>[4x]MKHHHHHHHHGGLVPRGSHG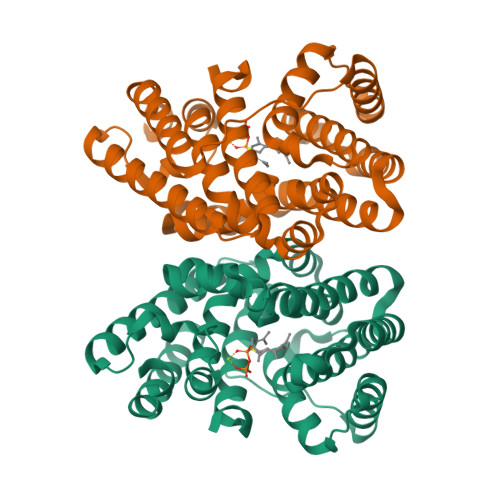GSEFMTTGLSTAGAQDIGRSSVRPYLEECTRRFQEMFDRHVVTRPTKVELTDAELREVIDDCNAAVAPLGKTVSDERWISYVGVVLWSQSPRHIKDMEAFKAVCVLNCVTFVWDDMDPALHDFGLFLPQLRKICEKYYGPEDAEVAYEAARAFVTSDHMFRDSPIKAALCTTSPEQYFRFRVTDIGVDFWMKMSYPIYRHPEFTEHAKTSLAARMTTRGLTIVNDFYSYDREVSLGQITNCFRLCDVSDETAFKEFFQARLDDMIEDIECIKAFDQLTQDVFLDLIYGNFVWTTSNKRYKTAVNDVNSRIQ> GMMKTIELEKEEIYCGNLLLVNKNYPLRDNNVKGLVPADI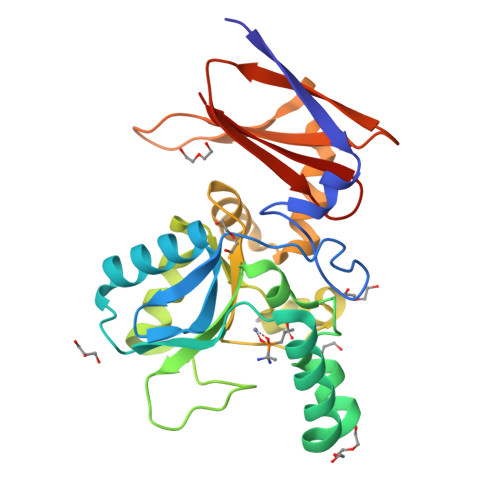RFPNILMKRDVANVLQLIFEKISAGNSIVPVSGYRSLEEQTAIYDGSLKDNGEDFTRKYVALPNHSEHQTGLAIDLGLNKKDIDFIRPDFPYDGICDEFRRAAPDYGFTQRYARDKEEITGISHEPWHFRYVGYPHSKIMQENGFSLEEYTQFIKAYLEDNKYLFEQAHRAEIEIYYVPAKDDKTLIKIPENCVYQISGNNIDGFVVTIWRKTDD>GPGGSPYLITGIPKDPKHPLPIRKDIDDWYLEQTSAGSNRIQLTLFVEALTVIQNRPLNDQLSYFRLAGIHGAPWTEWDGVPGGQKDSKGNPTGFAVHNNYTFPTWHRVYVTLYEQVIYEAMLDFIKQNVPQNGKADWENEAKQWRLPYWDFARFARHGHDNTQGDELRLPILVTMPMVKVLVPGQPGKQLSKPNPLYRFQMQTLMGTLERPYAITSQKTEEHGWSFDLPFDKCQSTTKYGLLENYNADVWADGGQNWLRANLALNEHPWYQNLDGWDSVPTLQDMTFRLLTTGGLNWGEFSSTRYDDKKEETQPKNNEQAPKNWMNLEAIHNNVHNWVGGFMFSRPGRHDLKLWGAGHMSSVPVAAYDPIFWLHHCNIDRLTAIWQTVNSGSWFNDDKSKVSKDDDLRPFHRFCEKTRKVVFFRSDDVKDWRSLNYDYAITKDASRIRKEIS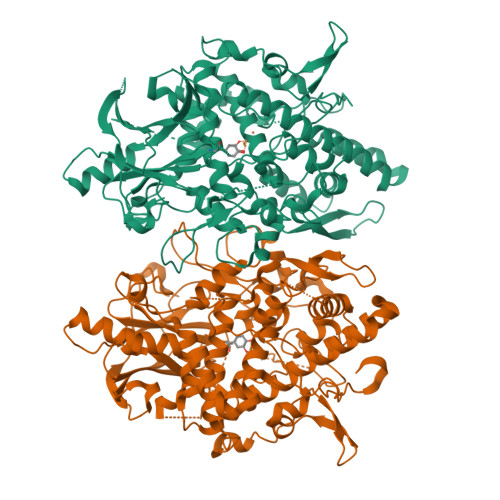DLYGQRTKEVYKDFGEEDYILSIRYSRYALGGKPFQINIFFGDVDGKDFYDARSQNFVGSVFNYSGSLEDSNCDKCAQQEQEGVLSVSQLPARLAVHYYKKQNKGEVPTPRYVVVNSQGKAEAEVKVEVALHKTEGTFYDAPARGGSDDYRRVADGKRAEVDDAYRA[2x]> MPVKEGQAKLWFSTKEEADAYDDKMISNIELKSQDYEDENFSPVFNRKTQEYFLEPSEKFKSDFAELLRPLRSLSFNQVVDRYVLIPPNHTFYRNWTYEKFLGGFGLSY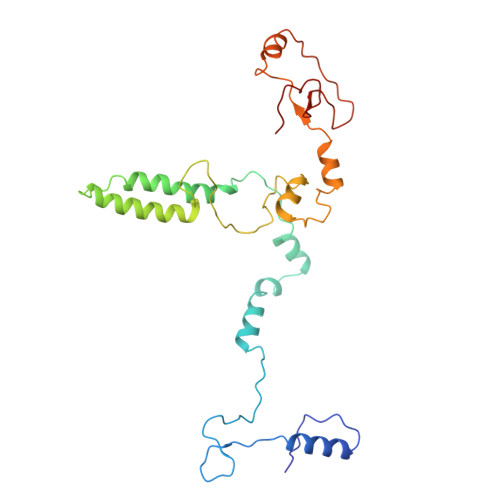LILRELPLRNFYARVFVMYAFAAKVLDHLGNPFPFSGHGQIVAAADRWNHWDVRCYDNVMKALKYIRIPTVQNNIPEATRWYGRQPGHLLRADTYWIPNLVSQRFAKHQPAHWDGTQNMPIFRLADPKHKDSYMVQFR> MVDAEMAAFGEAAPYLRKSEKERLEAQTRPFDLKKDVFVPDDKEEFVKATILSREGGKVTAETEHGKTVTVKEDQVLQQNPPKFDKIEDMAMLTFLHEPAVLYNLKERYASWMIYTYSGLFCVTINPYKWLPVYNAEVVAAYRGKKRSEAPPHIFSISDNAYQYMLTDRENQSILITGESGAGKTVNTKRVIQYFAVIAAIGDRSKKEQATGKGTLEDQIIQANPALEAFGNAKTVRNDNSSRFG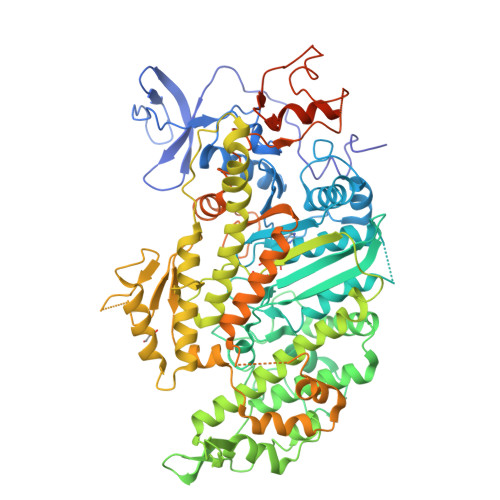KFIRIHFGATGKLASADIETYLLEKSRVIFQLKAERDYHIFYQILSNKKPELLDMLLITNNPYDYAFISQGETTVASIDDAEELMATDNAFDVLGFTTEEKNSMYKLTGAIMHFGNMKFKLKQREEQAEPDGTEEADKSAYLMGLNSADLLKGLCHPRVKVGNEYVTKGQNVQQVVYAKGALAKAVYERMFNWMVTRINATLETKQPRQYFIGVLDIAGFEIFDFNSFEQLCINFTNEKLQQFFNHHMFVLEQEEYKKEGIEWEFIDFGMDLQACIDLIEKPMGIMSILEEECMFPKATDMTFKAKLFDNHLGKSSNFQKPRNIKGKPEAHFSLIHYAGTVDYNIIGWLQKNKDPLNETVVDLYKKSSLKMLSSLFANYAGFDTPIEKGKGKAKKGSSFQTVSALHRENLNKLMTNLRSTHPHFVRCIIPNETKSPGVIDNPLVMHQLRCNGVLEGIRICRKGFPNRILYGDFRQRYRILNPAAIPEGQFIDSRKGAEKLLGSLDIDHNQYKFGHTKVFFKAGLLGLLEEMRDERLSRIITRIQAQSRGVLSRMEFKKLLERRDSLLIIQWNIRAFMGVKNWP Nicotinamide-N-methyltransferase (NNMT) is a cytosolic enzyme that catalyzes the transfer of a methyl group from S-adenosyl-methionine (SAM) to nicotinamide (Nam), yielding S-adenosyl-homocysteine (SAH) and 1-methylnicotinamide (MNam). NNMT is the major Nam-metabolizing enzyme, and systemic knockout in mice fully prevents MNam formation. As was described by Peng et al, NNMT possesses a class I AdoMet-dependent methyltransferase (MTase) core fold, comprising a central seven-stranded β-sheet, flanked on both sides by α-helices. In addition to the MTase core, there are two extra α-helices at the N-terminus, which, together with the β-hairpin Y203-S212, form a cap over the active site.

The crystal structure of the hNNMT complex with the HTS hit shows a very similar binding mode as for inhibitor. The NH group of inhibitor forms a hydrogen bond with the side chain of Tyr20 and also with the main chain oxygen atom of Leu164, and there are van der Waals contacts of the inhibitor with the side chains of Ser201 and Ser213. The 3-methyl-4-phenyl-pyrazole group of inhibitor (1) is located in the nicotinamide binding pocket which is occupied by (2) in the hNNMT complex of inhibitor (2); inhibitor (1) occupies both the SAH- and the Nam binding pockets. Based on the X-ray crystallographic data of our hits (1) and (2), the question arose as to whether the introduction of an appropriate 2-hydroxy-2-methyl-propionic carboxamide-based linker on (2) is able to transform our nicotinamide pocket binder into a true bisubstrate inhibitor.

>[4x]MGSSHHHHHHSSGLVPRGSMESGFTSKDTYLSHFNPRDYLEKYYKFGSRHSAESQILKHLLKNLFKIFCLDGVKGDLLIDIGSGPTIYQLLSACESFKEIVVTDYSDQNLQELEKWLKAAPAAFDWSPVVTYVCDLEGNRVKGPEKEEKLRQAVKQVLKCDVTQSQPLGAVPLPPADCVLSTLCLDAACPDLPTYCRALRNLGSLLKPGGFLVIMDALKSSYYMIGEQKFSSLPLGREAVEAAVKEAGYTIEWFEVISQSYSSTMANNEGLFSLVARKLSRPL>MANSPVSVFGLGAMGTALATQFLRKGHKTTVW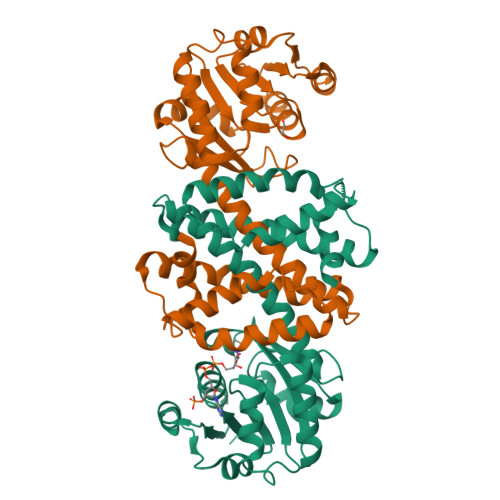NRTPAKAQPLIAIGASHAPTIDSAAAASSLLIICQLDKASVMQTLQQAPTAWAAKTIVDLTNGTPAHARETADWALAHGARYIHGGIMAVPFMIGQPDAMILYSGPAEVFEGVKDTLSVLGTNTYVGEDVGLASLHDLALLSGMYGLFSGFTHAVALVQSANIPAAGFVATQLIPWLTAMTQHLNLLATQVDEKDYGDGGSSLDMQAKAAPNILEASQAQGVSVELIQPIFKLIERRVEEGKGSEGLAALVGMIMK[2x]> AASCTTEDRREMQLMWGNVWSAQFTGRRIAIAQAVFKDLFANVPDAVGLFGAVKGDEVNSN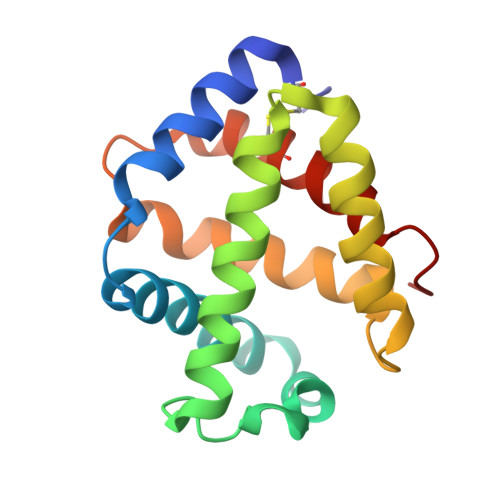EFKAHCIRVVNGLDSSIGLLSDPATLNEQLSHLATQHKARSGVTKGGFSAIAQSFLRVMPQVASCFNPDAWSRCFNRITTGMTEPLPA> AATSRDALPNTEASGPTHSKEIPALTAVETGATNPLVPSDTVQTRHVVQHRSRSESSIESFFARGACVTIMTVDNPASTTNKDKLFAVWKITYKDTVQLRRKLEFFTYSRFDMELTFVVTANFTETNNGHALNQVYQIMYVPPGAPVPEKWDDYTWQTSSNPSIFYTYGTAPARISVPYVGISNAYSHFYDGFSKVPLKDQSAALGDSLYGAASLNDFGILAVRVVNDHNPTKVTSKIRVYLKPKHIRVWCPRPPRAVAYYGPGVDYKDGTLTPLSTKDLTTY;> EACGYSDRVLQLTLGNSTITTQEAANSVVAYGRWPEYLRDSEANPVDQPTEPDVAACRFYTLDTVSWTKESRGWWWKLPDALRDMGLFGQNMYYHYLGRSGYTVHVQCNASKFHQGALGVFAVPEMCLAGDSNTTTMHTSYQNANPGEKGGTFTGTFTPDNNQTSPARRFCPVDYLLGNGTLLGNAFVFPHQIINLRTNNCATLVLPYVNSLSIDSMVKHNNWGIAILPLAPLNFASESSPEIPITLTIAPMCCEFNGLRNITLPRLQ;> GLPVMNTPGSNQYLTADNFQSPCALPEFDVTPPIDIPGEVKNMMELAEIDTMIPFDLSATKKNTMEMYRVRLSDKPHTDDPILCLSLSPASDPRLSHTMLGEILNYYTHWAGSLKFTFLFCGSMMATGKLLVSYAPPGADPPKKRKEAMLGTHVIWDIGLQSSCTMVVPWISNTTYRQTIDDSFTEGGYISVFYQTRIVVPLSTPREMDILGFVSACNDFSVRLLRDTTHIEQKA;> GAQVSSQKVGAHENSNRAY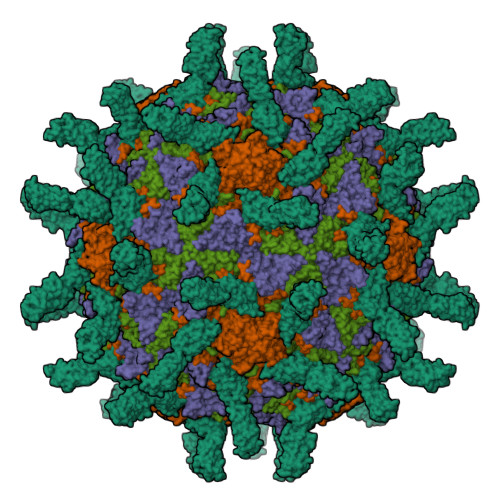GGSTINYTTINYYRDSASNAASKQDFSQDPSKFTEPIKDVLIKTAPMLN;> VVQAPTQVPGFLGDSVTLPCYLQVPNMEVTHVSQLTWARHGESGSMAVFHQTQGPSYSESKRLEFVAARLGAELRDASLRMFGLRVEDEGSYTCLFVTFPQGSRSVDIWLRVLAKPQNTAEVQKVQLTGEPVPMARCVSTGGRPPAQITWHSDLGGMPQTSQVPGFLSGTVTVTSLWILVPSSQVDGKQVTCKVEHESFEKPQLLTVSLTVYY Here, with the goal of combining the advantages of the P450 catalytic site geometry with the almost unlimited customizability of de novo protein design, we design a high-affinity heme-binding protein, dnHEM1, with an axial histidine ligand, a vacant coordination site for generating reactive intermediates, and a tunable distal pocket for substrate binding. We chose closed α helical solenoid repeat architectures as optimal structural solutions to the general porphyrin-based protein catalyst design challenge. These hyperstable proteins have large central cavities lined by side chains emanating from repeating structural units; the stability and structure of the fold are determined by hydrophobic packing interactions within the repeat units, and hence, the cavity lining residues are almost entirely reconfigurable. We sought to incorporate a heme-binding site within the central cavity of the toroid, with a proximal histidine ligand directly coordinating the iron atom of the cofactor, the distal site open for catalysis, and sufficient non-polar and hydrogen bonding side chain–cofactor interactions at the base and edges of the binding pocket to hold the heme in place without obstructing the free coordination site or interfering with potential substrate binding.

A 1.6 Å X-ray crystal structure of dnHEM1 reveals excellent agreement to the design model with key features programmed as intended. To aid with structure determination, the surface of the protein was desymmetrized by introducing two mutations K29W and K165Y. The heme cofactor is positioned as designed but adopts a flipped conformation, which alters the relative positioning of the heme vinyl and methyl substituents, but preserves the positioning of the heme propionates. Similar flipped heme orientations have previously been observed in natural and engineered heme proteins. The propionate groups interact with a network of polar residues (K15, S46, N50, R190). The heme iron is coordinated by His148 as designed, which in turn forms a hydrogen bond with the backbone carbonyl oxygen of Ile144. The open coordination site is occupied by an exogenous imidazole in the dnHEM1 crystal structure. Overall, the crystal structure shows that we were successful in achieving our design goals; the heme is held in place by numerous polar and hydrophobic side chain–cofactor interactions, and the heme iron is coordinated on one side by a designed histidine and, on the other, by a small molecule from a solution that occupies a central binding cavity. Arg43 in the distal pocket of dnHEM1 sits in a similar position, relative to the heme cofactor, to a conserved catalytic arginine found in natural peroxidases. The crystal structure of dnHEM1 demonstrates the attainment of our design goal: the creation of high-affinity heme-binding proteins with an open coordination site adjacent to a large reconfigurable substrate binding cavity.

> MVSLDQAILILVVAAKLGTTVEEAVKRALWLKTKLGVSLDQALRILSAAANTGTTVEEAVKRALKLKTKLGVSLEAALAILSAAAQLGTTVEEAVKRALKLKTKLGVDLETAALALLTAAKLGTTVEEAVKRALKLKTKLGVSLIEALHILLTAAVLGTTVEEAVYRALKLKTKLGVSLLQAAAILILAARLGTTVEEAVKRALKLKTKLGGGSGGSHHWGSGSHHHHHH> MRGSHHHHHHGSPYNVMIVDDAAMMRLYIASFIKTLPDFKVVAQAANGQEALDKLAAQ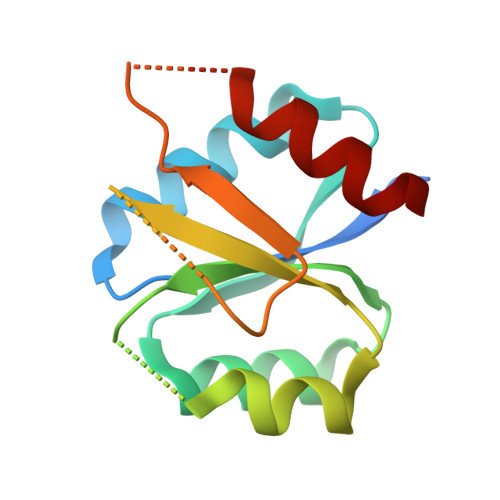PNVDLILLNIEMPVMDGMEFLRHAKLKTRAKICMLASVAVSGSPHAARARELGADGVVAKPSGTVSHDLEEKTGGELARTMRTLMAA> AMPFEIEVLLPGELSPAETSALQKCEGKIITFSTLRHRASLVDIALSSYYINGAPPDTLSLLEAYRMRFAAVITRVIPGKLLAHAIGVGTPTPGLFIQNTSPVDLCNGDYICLLPPVYGS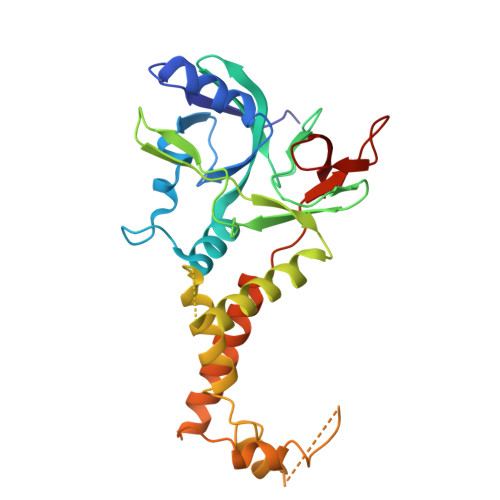ADSIRLDSVGLEIVFPLTIPQTLMREIIAKVVARAVEDLNLMFSINEGCLLILALIPRLLALLIPRLLALVTREAAQLIHPEAPMLMLPIYETISSWISTSSRLGDTLGTRAILRVCVFDGPSTVHPGDRTAVIQV>[2x]MCEQGVSYYNSQELKCCKLCKPGTYSDHRCDKYSDTICGHCPSDTFTSIYNRSPWCHSCRGPCGTNRVEVTP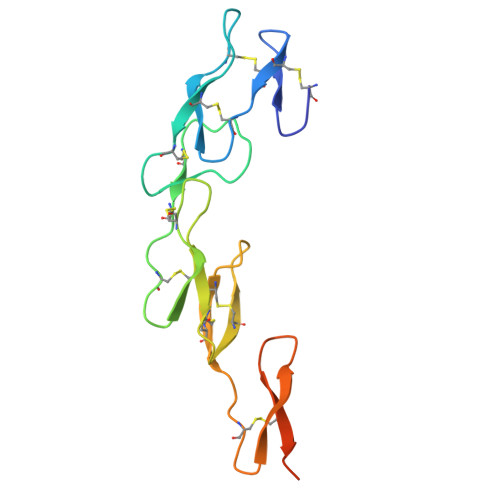CTPTTNRICHCDSNSYCLLKASDGNCVTCAPKTKCGRGYGKKGEDEMGNTICKKCRKGTYSKTGHHHHHH> GSHMKNATFYLLDNDTTVDGLSAVEQLVCEIAAERWRSGKRVLIACEDEKQAYRLDEALWARPAESFVPHNLAGEGPRGGAPVEIAWPQKRSSSRRDILISLRTSFADFATAFTE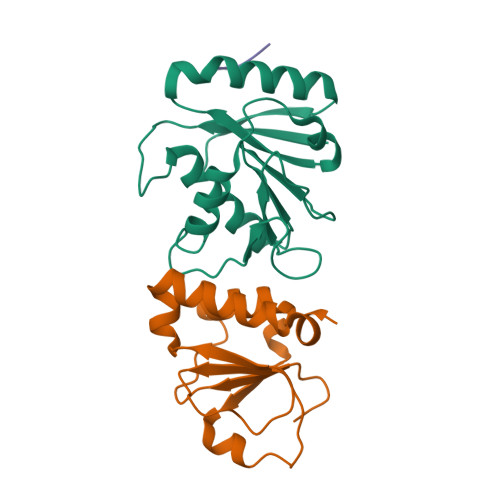VVDFVPYEDSLKQLARERYKAYRVAGFNLNTATWK;> MGTSRRDWQLQQLGITQWSLRRPGALQGEIAIAIPAHVRLVMVANDLPALTDPLVSDVLRALTVSPDQVLQLTPEKIAMLPQGSHCNSWRLGTDEPLSLEGAQVASPALTDLRANPTARAALWQQICTYEHDFFPRND;> WDIPF>SNAMTLEWEEFLDPYIQAVGELKIKLRGIRKQYRKQNKHSPIEFVTGRVKPIESIKEKMARRGITYATLEHDLQDIAGLRVMVQFVDDVKEVVDILHKRQDMRIIQERDYITHRKASGYRSYHVVVEYTVDTINGAKTILAEIQIRTLAMNFWATIEHSLNYKYQGDFPDEIKKRLEITARIAHQLDEEMG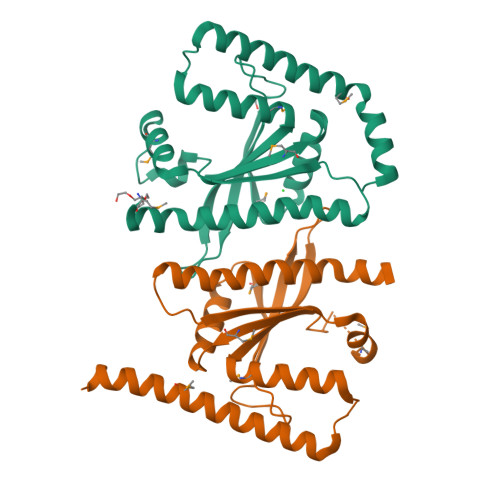EIRDDIQEAQALFDPLSRKLNDGVGNSDDTDEEYR[2x]>MKEVGSHFDDFVTNLIEKSASLDNGGCALTTFSVLEGEKNNHRAKDLRAPPEQGKIFIARRSLLDELLEVDHIRTIYHMFIALLILFILSTLVVDYIDEGRLVLEFSLLSYAFGKFPTVVWTWWIMFLSTFSVPYFLFQHWATGYSKSSHPLIRSLFHGFLFMIFQIGVLGFGPTYVVLAYTLPPASRFIIIFEQIRFVMKAHSFVRENVPRVLNSAKEKSSTVPIPTVNQYLYFLFAPTLIYRDSYPRNPTVRWGYVAMKFAQVFGCFFYVYYIFERLCAPLFRNIKQEPFSARVLVLCVFNSILPGVLILFLTFFAFLHCWLNAFAEMLRFGDRMFYKDWWNSTSYSNYYRTWNVVVHDWLYYYAYKDFLWFFSKRFKSAAMLAVFAVSAVVHEYALAVCLSFFYPVLFVLFMFFGMAFNFIVNDSRKKPIWNVLMWTSLFLGNGVLLCFYSQEWYARQHCPLKNPTFLDYVRPRSWTCRYVF[2x]

SOAT catalyzes the reaction between long chain fatty acyl-CoA and intracellular cholesterol to form the more hydrophobic cholesteryl ester, which is then stored in lipid droplets within the cell or transported in secreted lipoprotein particles to other tissues that need cholesterol. Previous studies have shown that SOAT1 is an ER-localized multi-transmembrane protein that is evolutionary conserved from yeast to humans. SOAT1 is the founding member of the membrane-bound O-acyltransferase (MBOAT) enzyme family, which transfers the acyl chain onto various substrates, including lipids, peptides and small proteins. Each hSOAT1 subunit is composed of nine transmembrane helices, which is consistent with previous prediction based on the biochemical data.

To overcome the conformational heterogeneity in the tetrameric hSOAT1 sample, the functional dimer construct (hSOAT1 66–550) was expressed and purified. The protein was reconstituted into the nanodisc in the presence of inhibitor CI-976. Subsequent 3D reconstruction generated a 3.5 Å cryo-EM map, which allowed the model to be built de novo. A strong extra non-protein density was found in the central cavity and the size and shape of the density matched that of the inhibitor CI-976, which was included during cryo-EM sample preparation. The large trimethoxyphenyl head of CI-976 is sandwiched between the catalytic residue H460 on M7, and residues N421 as well as W420 on the αD-αE loop, all of which are crucial for the catalytic activity of hSOAT1. The head of CI-976 also interact with Y416 and Y417 on αD. The elongated dodecanamide tail of CI-976 extends in the cavity and interacts with L377 on M6 and L515 on M9. In accordance with our assignment of CI-976, mutations of CI-976 interaction residues, N421A, H460A and H460N greatly diminished the enhancement effect of CI-976 on the thermostability of hSOAT1 dimer. The binding position of CI-976, right in the catalytic center, suggests that it inhibits the enzyme by precluding the loading of substrate into the catalytic center. This is consistent with the competitive behavior of CI-976.>SNAMEEKFLEFGGNQICLCSWGSPEHPVVLCIHGILEQGLAWQEVALPLAAQGYRVVAPDLFGHGRSSHLEMVTSYSSLTFLAQIDRVIQELPDQPLLLVGHSMGAMLATAIASVRPKKIKELILVELPLPAEESKKESAVNQLTTCLDYLSSTPQHPIFPDVATAASRLRQAIPSLSEEFSYILAQRITQPNQGGVRWSWDAIIRTRSILGLNNLPGGRSQYLEMLKSIQVPTTLVYGDSSKLNRPEDLQQQKMTMTQAKRVFLSGGHNLHIDAAAALASLILTS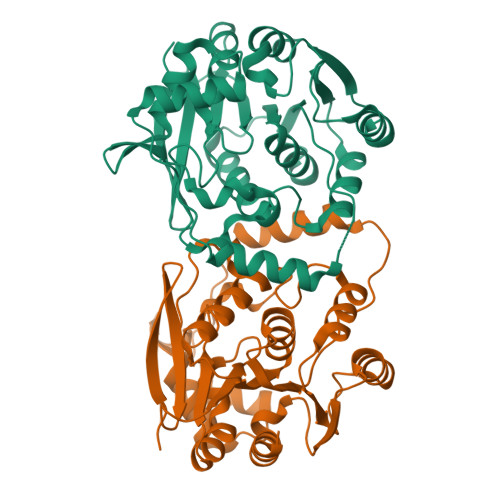[4x]> MSGTANSRRKEVLRVPVIDLNRVSDEEQLLPVVRAILL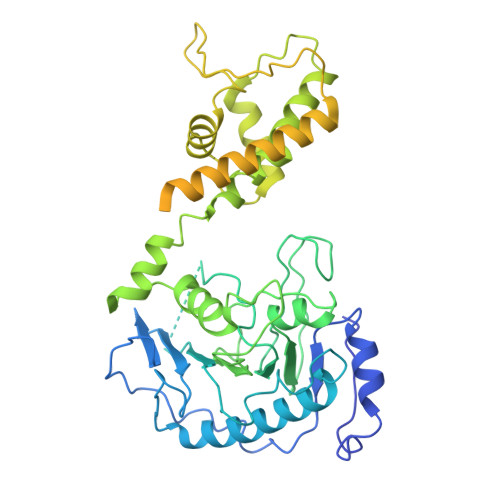QHDTFLLKNYANKAVLDALLAGLTTKDLPDTSQGFDANFTGTLPLEDDVWLEQYIFDTDPQLRFDRKCRNESLCSIYSRLFKLGLFFAQLCVKSVVSSAELQDCISTSHYATKLTRYFNDNGSTHDGADAGATVLPTGDDFQYLFERDYVTFLPTGVLTIFPCAKAIRYKPSTMATTDNSWVSIDEPDCLLFHTGTLLARWSQGMHTTSPLQIDPRANIVSLTIWPPLTTPISSKGEGTIANHLLEQQIKAFPKVAQQYYPRELSILRLQDAMKFVKELFTVCETVLSLNALSRSTGVPPELHVLLPQISSMMKRKIVQDDILKLLTIWSDAYVVELNSRGELTMNLPKRDNLTTLTNKSRTLAFVERAESWYQQVIASKDEIMTDVPAFKINKRRSSSNSKTVLSSKVQTKSSNANALNNSRYLANSKENFMYKEKMPDSQANLMDRLRERERRSAALLSQRQKRYQQFLAMKMTQVFDILFSLTRGQPYTETYLSSLIVDSLQDSNNPIGTKEASEILAGLQGILPMDISVHQVDGGLKVYRWNSLDKNRFSKLLQIHKSKQQD> MGSSHHHHHHSQDLEVLFQGPGSVATDELTGLFNRRHFMRMASRALEDLLPNRQHGLALIDLDHFKRINDRHGHAAGDRVLQTFAAVARSCLRDGDVLARYGGEEFVLLLPHADAEQLESCCERLRLA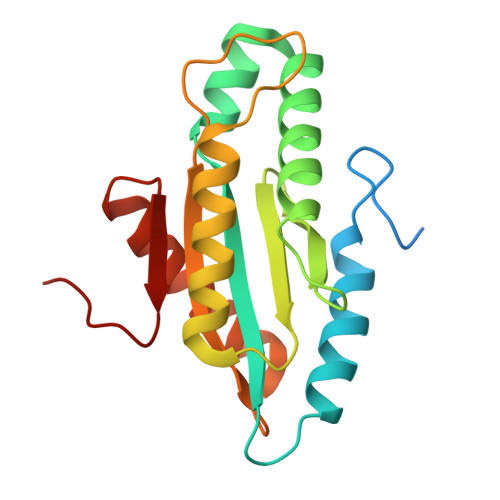FQQAEPVGVTVDTLSLSVGMTLLYADDDLDEALQRADQALYRAKRGGRNRCDATWEVTSA>[4x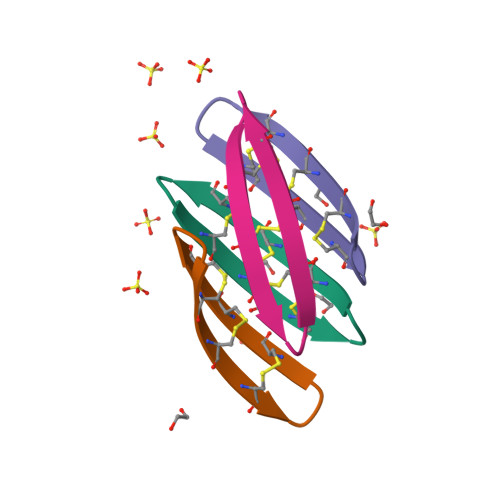]GVCRCVCRRGVCRCVCRR> MGSSHHHHHHSQDPMGAERRLLSIKEAFRLAQQPHQNQAKLVVALSRTYRTMDDKTVFHEEFIHYLKYVMVVYKREPAVERVIEFAAKFVTSFHQSDMEDDEEEEDGGLLNYLFTFLLKSHEANSNAVRFRVCLLINKLLGSMPENAQIDDDVFDKINKAMLIRLKDKIPNVRIQAVLALSRLQDPKDDECPVVNAYATLIENDSNPEVRRAVLSCIAPSAKTLPKIVGRTKDVKEAVRKLAYQVLAEKVHMRAMSIAQRVMLLQQGLNDRSDAVKQAMQKHLLQGWLRFSEGNILELLHRLDVENSSEVAVSVLNALFSITPLSELVGLCKNNDGRKLI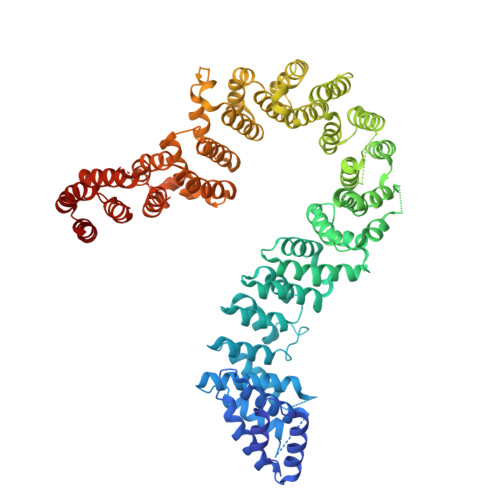PVETLTPEIALYWCALCEYLKSKGDEGEEFLEQILPEPVVYADYLLSYIQSIPVVNEEHRGDFSYIGNLMTKEFIGQQLILIIKSLDTSEEGGRKKLLAVLQEILILPTIPISLVSFLVERLLHIIIDDNKRTQIVTEIISEIRAPIVTVGVAETLQKCLILCYELLKQMSISTGLSATMNGIIESLILPGIISIHPVVRNLAVLCLGCCGLQNQDFARKHFVLLLQVLQIDDVTIKISALKAIFDQLMTFGIEPFKTKKIKTLHCEGTEINSDDEQESKEVEETATAKNVLKLLSDFLDSEVSELRTGAAEGLAKLMFSGLLVSSRILSRLILLWYNPVTEEDVQLRHCLGVFFPVFAYASRTNQECFEEAFLPTLQTLANAPASSPLAEIDITNVAELLVDLTRPSGLNPQAKTSQDYQALTVHDNLAMKICNEILTSPCSPEIRVYTKALSSLELSSHLAKDLLVLLNEILEQVKDRTCLRALEKIKIQLEKGNKE>MQRREFLKLSALGVGAMALRGSGPAKALKAPWYAQEVKSVYQICEGCFWRCGIVAHAVGNRVYKVEGYEANPKSRGRLCPRGQGAPQTTYDPDRLKRPLIRVEGSQRGEGKYRVATWEEALD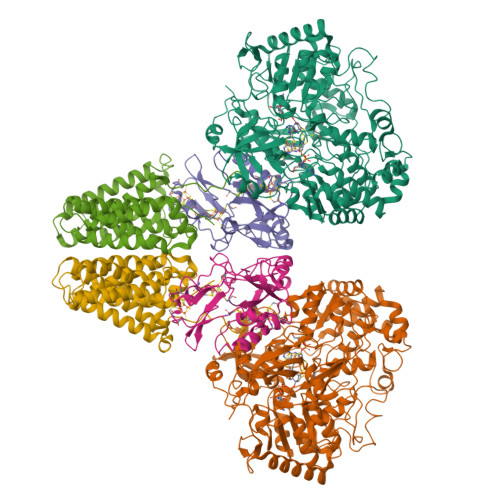HIAKKMLEIREKYGPEAIAFFGHGTGDYWFVDFLPAAWGSPNAAKPSVSLCTAPREVASQWVFGRPIGGHEPIDWENARYIVLIGHHIGEDTHNTQLQDFALALKNGAKVVVVDPRFSTAAAKAHRWLPIKPGTDTALLLAWIHVLIYEDLYDKEYVAKYTVGFEELKAHVKDFTPEWAEKHTEIPAQVIREVAREMAAHKPRAVLPPTRHNVWYGDDTYRVMALLYVNVLLGNYGRPGGFYIAQSPYLEKYPLPPLPLEPAAGGCSGPSGGDHEPEGFKPRADKGKFFARSTAIQELIEPMITGEPYPIKGLFAYGINLFHSIPNVPRTKEALKNLDLYVAIDVLPQEHVMWADVILPEATYLERYDDFVLVAHKTPFIQLRTPAHEPLFDTKPGWWIARELGLRLGLEQYFPWKTIEEYLETRLQSLGLDLETMKGMGTLVQRGKPWLEDWEKEGRLPFGTASGKIELYCQRFKEAGHQPLPVFTPPEEPPEGFYRLLYGRSPVHTFARTQNNWVLMEMDPENEVWIHKEEAKRLGLKEGDYVMLVNQDGVKEGPVRVKPTARIRKDCVYIVHGFGHKAPLMRLAHGRGASDNYLQTRYKLDPISGGAGLRVNFVRLEKAERPRLPSLTGLAKRPFDERRM[2x];>MPRYAMAIDLSLCVGCAACAVACKMENEVPPGVFNLWIREREVGEYPNLVVEFRPEQCLHCENPPCVPVCPTGASYQTKDGLVLVDPKKCIACGACIAACPYDARYLHPAGYVSKCTFCAHRLEKGKVPACVETCPTYCRTFGDLEDPESPVAKALKAAERVDVLRPEQGTRPKLFYLNAPSKKGLTRESEVHHG[2x];>MAEFYGLPNAQEFWHWTNALHFVLVGLAGGVALLAALLHLKGDAEARRYTLYALMLIALDLFILWAESPARFRFTHIWLFLSFHPTSPIWWGAWGLGLGFLTGGLLYLGKGSQRALAWALLVFSLVALSYPGLALAVNLNRPLWNGLMAGLFPLTALVLALGLAALLKSPWALFPLRVLAGASLLLALLYPLTLPPEARGHLLEEAGFWYGLFLLLGLGTFWQERLAPWAGLLAAAGLRALLVLAGQWQGLGL[2x]>MWSHPQFEKASGTFYDVIEDYRHFDFAAYFAKVTDSDVRRILRQDRLSALDFLTLLSPQAEAYLEEMAQKAHRLTVQHFGRTMLLYTPLYLANYCVNQCVYCGFQLKNKLERKKLTLAEVEQEAQLIAATGLKHILILTGESRQHSPVSYIKDCVNILKKYFSSISIEIYPLTQEEYAELIGAGVDGLTIYQEVYNEEVYAEMHPAGPKRNYRFRLEAPERACQAGMRTVNIGALLGLNDWRQEAFFTGLHADYLQRRFPDVEVSISPPRMRPHLGGFPPRVVVSDQNLVQYVLAFRLFMPRSGITLSTRENGRLRDAMVRLGVTKMSAGSCTAVGGRSDQEAVGQFQISDERTVAEVAAMLYAQGYQPVYKDWQAL[2x]

2-iminoacetate synthase ThiH is a radical S-adenosyl-L-methionine (SAM) L-tyrosine lyase and catalyzes the L-tyrosine Cα–Cβ bond break to produce dehydroglycine and p-cresol while the radical SAM L-tryptophan lyase NosL cleaves the L-tryptophan Cα–C bond to produce 3-methylindole-2-carboxylic acid. Dehydroglycine (DHG), also termed 2-iminoacetate, is a key precursor in the bacterial biosynthesis of the thiazole ring that constitutes the core of TPP. The radical SAM domain includes residues 71 to 356 and corresponds to a full (βα)8 triose-phosphate isomerase-like fold flanked by N- and C-terminal stretches.

TcThiH was incubated with its substrate L-tyrosine, 5´-deoxyadenosine (5´-dA) and methionine as mimics of the SAM cleavage products prior to crystallization. Brownish prism-shaped crystals that diffracted to 1.27 Å resolution were obtained. Inspection of the electron density map indicates features that can be best modeled as 5´-dA, L-methionine bound to the radical SAM [Fe4S4]-cluster and L-tyrosine. The amino nitrogen atom interacts with Nη2 of the strictly conserved residue R300 and points toward the C5´-atom of 5´-dA, supporting a direct hydrogen-atom abstraction from that position by the 5´-dA• species. The carboxyl moiety is sandwiched between the strictly conserved residue R300 Nη1- and E158 Oε1-atoms. These unexpected interactions suggest an unusual protonation state to avoid electrostatic repulsions between the amino and guanidinium groups on the one hand and the two carboxyl moieties on the other hand. The phenol ring sits in a narrow hydrophobic pocket while the phenol oxygen atom establishes four polar interactions with the hydroxyl groups of the strictly conserved residues T299, S318 and S321, in addition to the main-chain nitrogen amide of residue T299, hence defining a square pyramidal geometry supporting anion-dipole interactions instead of hydrogen-bonding. We have also performed a 250-ns molecular dynamics (MD) simulation of L-Tyr bound TcThiH at the optimal bacterial growth temperature (60 °C). Both approaches show that only the phenolate-containing models were able to reproduce the phenol oxygen atom interactions with the protein observed in the crystal structure, hence supporting deprotonation of the phenol upon L-tyrosine binding. Therefore, upon binding, L-tyrosine would be fully deprotonated, likely corresponding to NH2-CH-(Ph-O−)(COO−). In addition, as predicted when we solved the L-tryptophan bound NosL structure, this new structure confirms that 5´-dA• attacks the amino group of L-tyrosine in ThiH.>[4x]MSKLAIIAGDGIGPEVTAEAVKVLDAVVPGVQKTSYDLGARRFHATGEVLPDSVVAELRNHDAILLGAIGDPSVPSGVLERGLLLRLRFE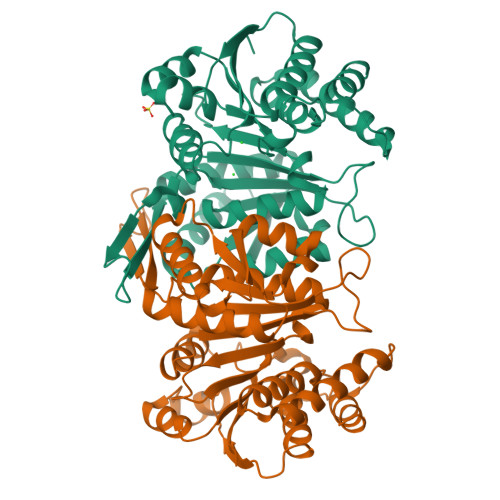LDHHINLRPARLYPGVASPLSGNPGIDFVVVREGTEGPYTGNGGAIRVGTPNEVATEVSVNTAFGVRRVVADAFERARRRRKHLTLVHKTNVLTFAGGLWLRTVDEVGECYPDVEVAYQHVDAATIHMITDPGRFDVIVTDNLFGDIITDLAAAVCGGIGLAASGNIDATRANPSMFEPVHGSAPDIAGQGIADPTAAIMSVALLLSHLGEHDAAARVDRAVEAHLATRGSERLATSDVGERIAAAL>MYNFDEIIDRRNTNAMNTDGFRSYIFHADENMKFPYKDEEFIRMWVADMEFATPQVIIDGIKERLDKRIFGYTKIFSNDYYNAFSDWCQRRYGWNFEKKHLVMSNGIIPALYELVQYICKKDEKVLFLTPSYAYFKYAADFSNRTPICSDLIDNDGYYTIDFEDFEKKAADEKTTLFILCNPHNPTGRVWKEEELKKLGKICEKYDVWVISDEIHCDLLRCDKQHIPLAKLFPNYKRIITCMAPSKTFNLAGLMISNVIIPDDNLREVWLSKHYNFDNPLSVAGAQAAYEKGEDWLKELQKYLDKNFEFTKEYLNKNLPKAKFKISEATYLAWVNLEEYFDKTENLPIFFANKAGVLLEGGNMFV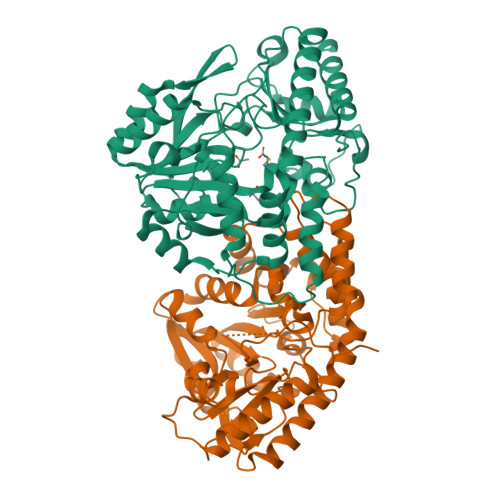QNSDCFIRLNLACPKSILEKGLKRICKAVNEKHHHHHH[2x]> AYPETVDWRTKGAVTGIKSQGDCGASYAFSAMGALEGINALATGKLTYLSEQNIIDCSVPYGNHGCKGGNMYVAFLYVVANEGVDDGGSYPFRGKQSSCTYQEQYRGASMSG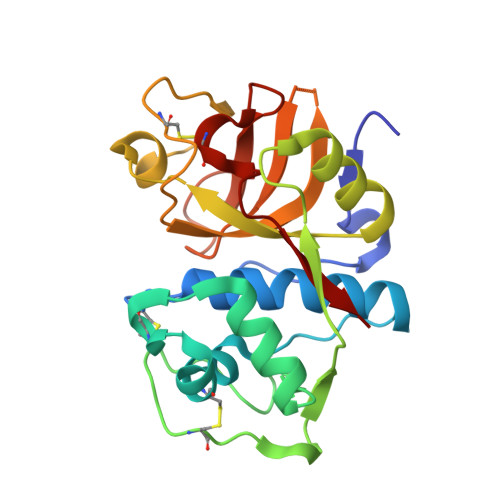SVQINSGSESDLEAAVANVGPVAVAIDGESNAFRFYYSGVYDSSRCSSSSLNHAMVITGYGISNNQEYWLAKNSWGENWGELGYVKMARNKYNQCGIASDASYPTL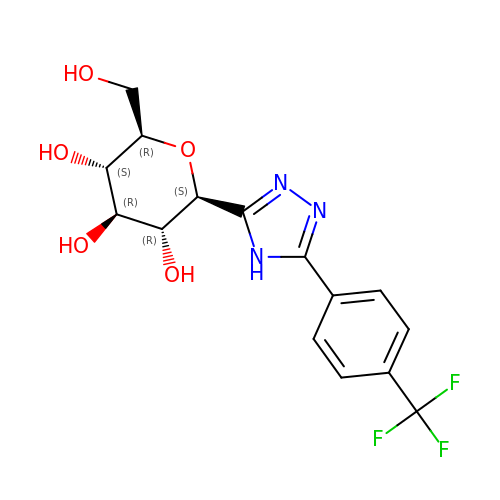(2~{R},3~{S},4~{R},5~{R},6~{S})-2-(hydroxymethyl)-6-[5-[4-(trifluoromethyl)phenyl]-4~{H}-1,2,4-triazol-3-yl]oxane-3,4,5-triol | C15 H16 F3 N3 O5 | DRGPMAPBLAZFLD-RMPHRYRLSA-N>[64x]MGI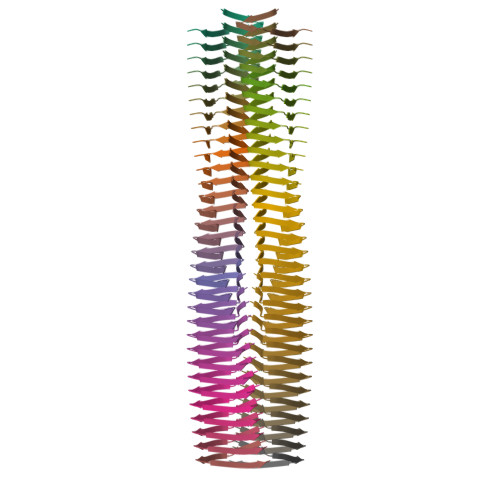IAGIIKVIKSLIEQFTGK> MRKPRHITALLFCLLTSLTSVADNHSEQTLYQLMSERLALMPEVAKYKWHHNLPIEDLAREAMVLERTVSRTTVLDPIHTKTFFGLQMTAAKAIQANVFQSLTNTDVVASDVRSLNDDLRPKLTLLGDQIIEQLLISYQNGTPLNRAHFDAHFAHFELNPQIKDGLFKSLELVLTPPNLDPRDTLARLEKDKTLRVGVTLDYEPFSYQDNEGNRAGIDIELATALAKEFGYRIVWVKTSWPTLMADAEDNLFDIALSGISITAQRQHRMMFSAPYHTGGKTAIGRCSSVDELNTLALIDRAETRIIVNPGGTNERFVRSALTNASIRIHPDNRTIFNELVSGTADAMFTDSIEAQLQATKHPSLCVLLDQPLTFQQKGILLQPDPELKKRIDTWLLDYLSSHDVSALFSKHGVDPDLEHHHHHH

Chorismate mutase (CM) and cyclohexadienyl dehydratase (CDT) catalyze two subsequent reactions in the intracellular biosynthesis of l-phenylalanine (Phe). Here, we report the discovery of novel and extremely rare bifunctional fusion enzymes, consisting of fused CM and CDT domains, which are exported from the cytoplasm. In γ-proteobacterial fusion enzymes, the CM domain is N-terminal to the CDT domain, whereas the order is inverted in β-Proteobacteria. The fusion enzymes of Aequoribacter fuscus, Janthinobacterium sp. HH01, and Duganella sacchari were crystallized and their structures refined to 1.6, 1.7, and 2.4 Å resolution, respectively.

To investigate the relative locations of the active sites within a single polypeptide, ∗AfCMCDT, ∗JbCDTCM, and ∗DsCDTCM were crystallized, and their structures solved and refined to 1.6, 1.7, and 2.4 Å resolution, respectively, and Rfree/Rwork values of 24.8/20.5%, 24.3/19.9%, and 25.8/23.0%. Like ∗MtCM, the CM domains of ∗AfCMCDT, ∗JbCDTCM, and ∗DsCDTCM form six-helix bundles with a single active site in the N-terminal moiety. In ∗AfCMCDT, representing the ∗CMCDT topology, the presumed substrate access to the CDT domain faces away from the expected product exit site of the CM domain, with a distance of 35 Å between active sites. A full structural assessment of the domain interface in ∗AfCMCDT is precluded by the poorly resolved linker region. In fact, there is ambiguous electron density for residues Pro177-Asp180. This may suggest a more flexible connection of the CM and CDT domains for ∗AfCMCDT than for the topological counterparts ∗JbCDTCM and ∗DsCDTCM, for which the linker regions are clearly resolved. Still, residues Asp164 and Lys168 from H6 of the CM domain of ∗AfCMCDT interface extensively with the CDT domain. There is no indication of dimer formation of ∗AfCMCDT; however, we noted a right-hand shoulder of the main peak, which could be due to conformational isomers, e.g., due to partial unfolding. The coupled CM+CDT reactions showed that equimolar concentrations of the active-site KO variants ∗AfCMCDT and ∗AfCMCDT complemented each other perfectly and reached a catalytic activity (kcat = 2.8 ± 0.2 s−1, Km = 9.2 ± 1.5 μM, kcat/Km = 3.0 ± 0.7 × 105 M−1 s−1) that coincides, within experimental error, with that of wild-type ∗AfCMCDT. This result directly suggests that the enzyme fusion does not provide a catalytic benefit.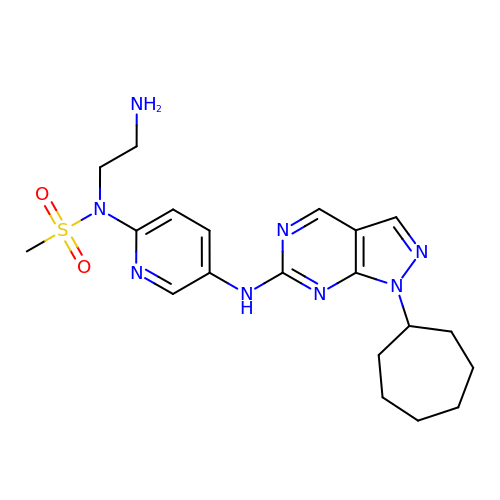N-(2-aminoethyl)-N-{5-[(1-cycloheptyl-1H-pyrazolo[3,4-d]pyrimidin-6-yl)amino]pyridin-2-yl}methanesulfonamide | C20 H28 N8 O2 S | SZKRTTIHILIRKD-UHFFFAOYSA-N>[4x]KETAAAHFEHQHMDSSTSAASSSNYCNQMMKSRNLTKDRCKPVNTFVHESLADVQAVCSQKNVACKNGQTNCYQSYSTMSITD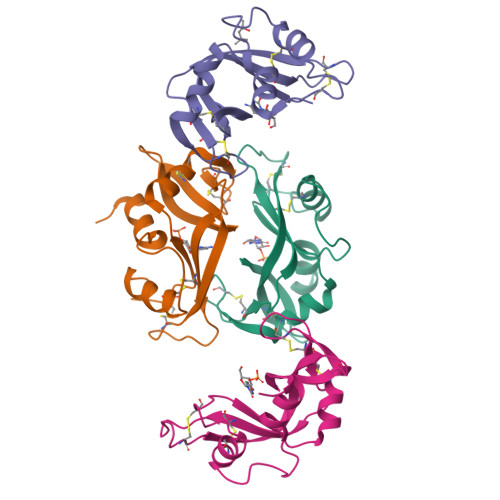CRETGSSKYPNCAYKTTQANKHIIVACEGNPYVPVHFDASV> HCRLDKSNFQQPYITNRTFMLAKEASLADQNTDVRLIGEKLFHGVSMSERCYLMKQVLQFTLEEVLFPQSDRFQPYMQEVVPFLARLSNRLSTCHIEGDDLHIQRNVQKLKDTVKKLGESGEIKAIGELDLLFM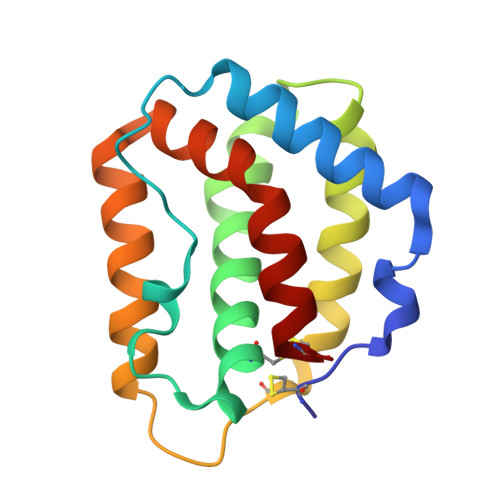SLRNACI>[4x]TNLVAEPFAKLEQDFGGSIGVYAMDTGSGATVSYRAEERFPLCSSFKGFLAAAVLARSQQQAGLLDTPIRYGKNALVPWSPISEKYLTTGMTVAELSAAAVQYSDNAAANLLLKELGGP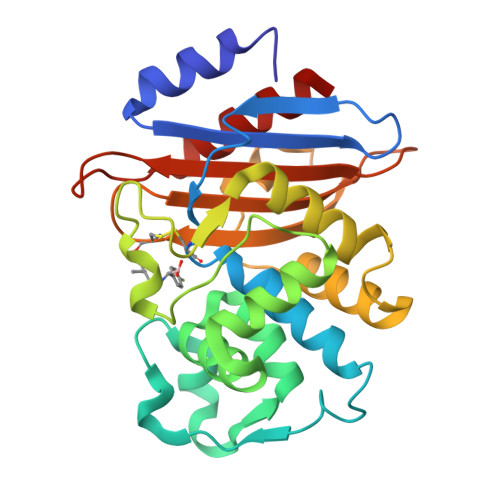AGLTAFMRSIGDTTFRLDRWELELNSAIPGDARDTSSPRAVTESLQKLTLGSALAAPQRQQFVDWLKGNTTGNHRIRAAVPADWAVGDKTGTCGVYGTANDYAVVWPTGRAPIVLAVYTRAPNKDDKHSEAVIAAAARLALEGLG> VPRGSHMSSGKTCPTSEVSPACYANQWETTFPPSDIKITGATWVQDNIYDVTLSYEAESLELENLTELKIIGLNSPTGGTKLVWSLNSKVYDIDNPAKWTTTLRVYTKSSADDCYVEMYPFQIQVDWCEAGASTDGCSAWKWPKSYDYDIGCDNMQDGVSRKHHPVYKWPKKCSSNCGVEPTT

Flo11-type adhesins are of interest in the context of kin discrimination, because Flo11 from the budding yeast Saccharomyces cerevisiae (ScFlo11) confers cell aggregation by homotypic protein-protein interaction (Bayly et al., 2005; Goossens and Willaert, 2012; Kraushaar et al., 2015; Barua et al., 2016). Moreover, Flo11 confers the formation of diverse multicellular growth forms representing cooperative communities including biofilms, invasive filaments or adhesive aggregates. The structural and mutational analysis of different Flo11A domains demonstrates that homotypic Flo11A-Flo11A interactions depend on evolutionary conserved aromatic residues, which form two bands at the Flo11A surface. By employing biophysical (SCFS), cell aggregation (QCAM) measurements and competitive biofilm assays, we demonstrate that Flo11-type domains from diverse yeasts confer efficient cell-cell adhesion at single cell level and in populations in homotypic configurations and are able to efficiently discriminate between kin and non-kin variants in heterotypic situations in vivo.

Given our finding that Flo11A-mediated cellular adhesion appears to be well-conserved in Saccharomycetales, we wondered to which extent structures are conserved. Therefore, the crystal structure of Flo11A from K. pastoris (KpFlo11A), a variant from the family of Phaffomycetaceae, was determined at a resolution of 1.40 Å. Despite a sequence identity between KpFlo11A and ScFlo11A of only 32%, their overall structures showed a high degree of similarity with an r.m.s.d. of 1.01 Å for 102 Cα atoms after superposition. The core motif of KpFlo11A, the FNIII domain, showed the highest degree of similarity (0.70 Å for 61 Cα atoms derived from the β-sheet), whereas the neck-like subdomain and the apical regions deviated from ScFlo11A. The surface of KpFlo11A exposed 6 tryptophans and nine tyrosines that cluster in two bands, which were similar but not identical to the aromatic bands of ScFlo11A. Also, both the KpFlo11A and ScFlo11A surfaces were quite rigid given the low thermal B factors found for their surface-exposed aromatic residues. Thus, the core and aromatic surface patterns of even highly divergent Flo11A domains appeared to be conserved, explaining the functional conservation with respect to cellular adhesion. Similar to ScFlo11A, KpFlo11A is able to undergo homophilic interactions with a KD of 31.8 µM. We also measured possible heterophilic interactions between ScFlo11A and KpFlo11A, where we found a clearly decreased interaction with a KD of 121.1 µM. Thus, both ScFlo11A and KpFlo11A are competent for efficient homophilic interactions in vitro, but they are able to clearly discriminate between each other.> MWYLLWFVGILL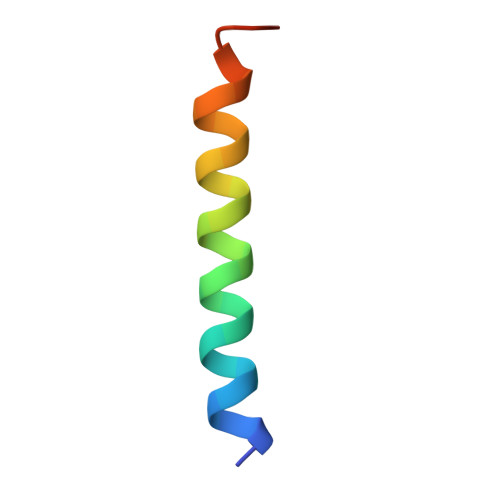MCSLSTLVLVWLDPRLKS>[4x]SELYRQSLEIISRYLREQATGAKDTKPMGRSGATSRKALETLRRVGDGVQRNHETAFQGMLRKLDIKNEDDVKSLSRVMIHVFSDGVTN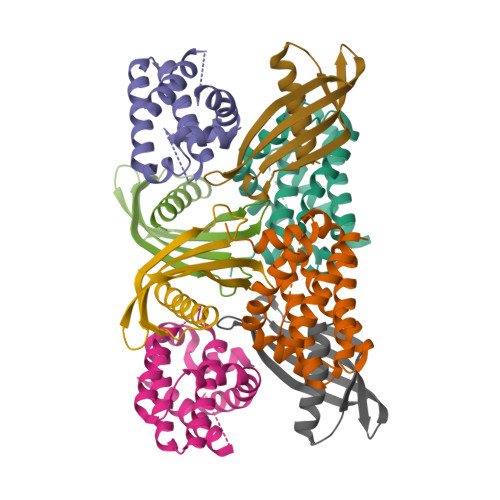WGRIVTLISFGAFVAKHLKTINQESCIEPLAESITDVLVRTKRDWLVKQRGWDGFVEFFHVEDLEGG;>[4x]SENSLEIEELARFAVDEHNKKENALLEFVRVVKAKEQMGVNPEEMQTMYYLTLEAKDGGKKKLYEAKVWVKWWWGFHIWDNFKELQEFKPV> MTEKKERIDVHAYLAEFDDIPGTRVFTAQRARKGYNLNQFAMSLMKAENRERFKADESAYLDEWNLTPAAKAAVLARDYNAMIDEGGNVYFLSKLFSTDGKSFQFAAGSMTGMTQEEYAQMMIDGGRS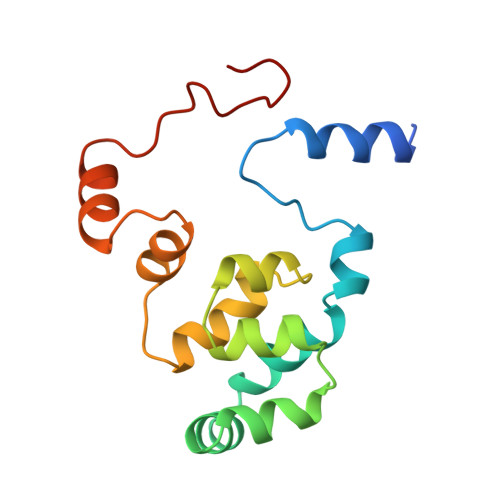PAGVRSIKGGY> ITVFSPDGRLFQVEYAREAVKRGATAIGIKC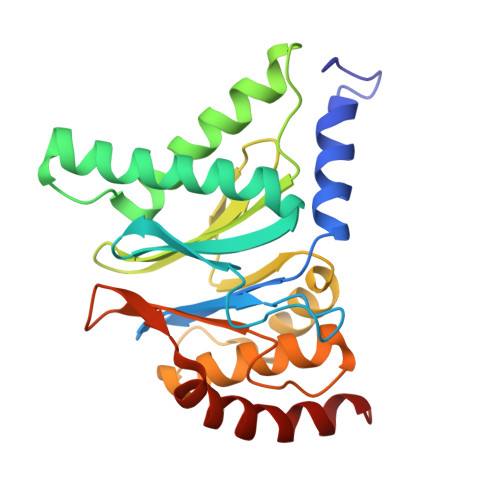KEGVILIADKRVGSKLLEADTIEKIYKIDEHICAATSGLVADARVLIDRARIEAQINRLTYDEPITVKELAKKICDFKQQYTQYGGVRPFGVSLLIAGVDEVPKLYETDPSGALLEYKATAIGMGRNAVTEFFEKEYRDDLSFDDAMVLGLVAMGLSIESELVPENIEVGYVKVDDRTFKEVSPEELKPYVERANERIRELLKK> MDMANQLLDELAHGNFSHLTLNLSQNGREIAILQKQLTGFDDKQLETFVEQHPAMPNDTRFKIMCTSFLNYARDVDPWSAWSSSDLIFEFYQCLINCLINDNAPHIEMLIPVATRETEFIINLAGKLDSFHLQLHTRSHQFLSHISSILSRLFNSIKPPRGNASSTNIPGKQRILLYLVNKLNNIYFRIESPQLCSNIFKNFQPKSMLAHFNEYQLDQQIEYRYLLGRYYLLNSQVHNAFVQFNEAFQSLLNLPLTNQAITRNGTRILNYMIPTGLILGKMVKWGPLRPFLSQETIDNWSVLYKHVRYGNIQGVSLWLRQNERHL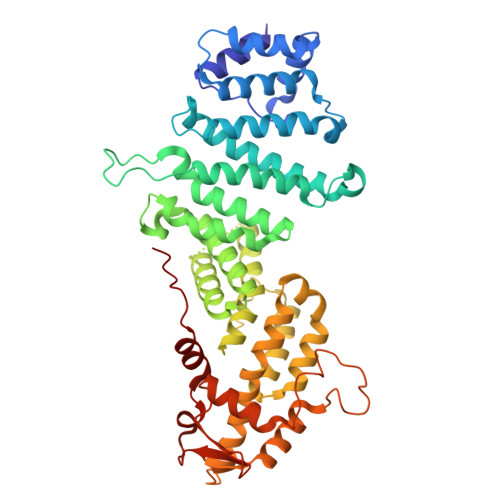CARQLLIVLLEKLPMVTYRNLIKTVIKSWTTEWGQNKLPYSLIERVLQLSIGPTFEDPGAQEITIYNGIHSPKNVENVLVTLINLGLLRANCFPQLQLCVVKKTTMIQEIVPPVNERITKMFPAHSHVLW> GSHMASFNGVSEAELLTKTLPDILTFNLDIVIIGIAPGLMAAYKGHHYPGPGNHFWKCLFMSGLSEVQLNHMDDHTLPGKYGIGFTN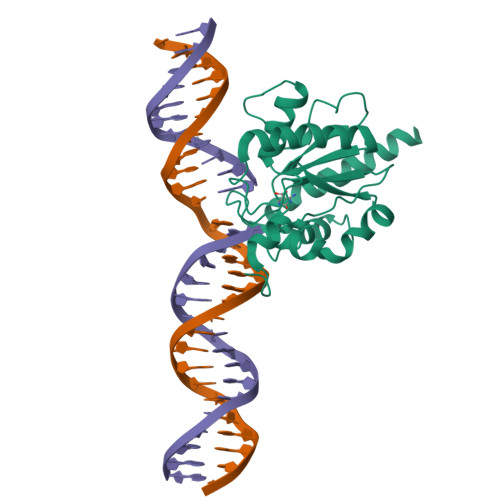MVERTTPGSKDLSSKEFREGGRILVQKLQKYQPRIAVFNGKCIYEIFSKEVFGVKVKNLEFGLQPHKIPDTETLCYVMPSSSARCAQFPRAQDKVHYYIKLKDLRDQLKGIERNMDV>MKVEEILEKALELVIPDEEEVRKGREAEEELRRRLDELGVEYVFVGSYARNTWLKGSLEIDVFLLFPEEFSKEELRERGLEIGKAVLDSYEIRYAEHPYVHGVVKGVEVDVVPCYKLKEPKNIKSAVDRTPFHHKWLEGRIKGKENEVRLLKGFLKANGIYGAEYKVRGFSGYLCELLIVFYGSFLETVKNARRWTRRTVIDVAKGEVRKGEEFFVVDPVDEKRNVAANLSLDNLARFVHLCREFMEAPSLGFFKPKHPLEIEPERLRKIVEERGTAVFAVKFRKPDIVDDNLYPQLERASRKIFEFLERENFMPLRSAFKASEEFCYLLFECQIKEISRVFRRMGPQFEDERNVKKFLSRNRAFRPFIENGRWWAFEMRKFTTPEEGVRSYASTHWHTLGKNVGESIREYFEIISGEKLFKEPVTAELCEM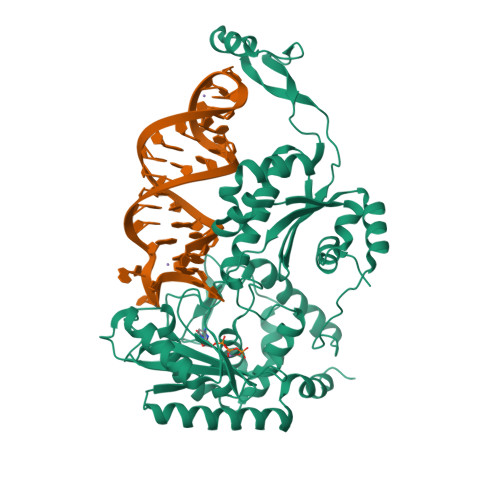MGVKDSNSSSVDKLAAALEHHHHHH[2x]>[2x]MKEYHIDEEVGFALPNPQENLPDFYN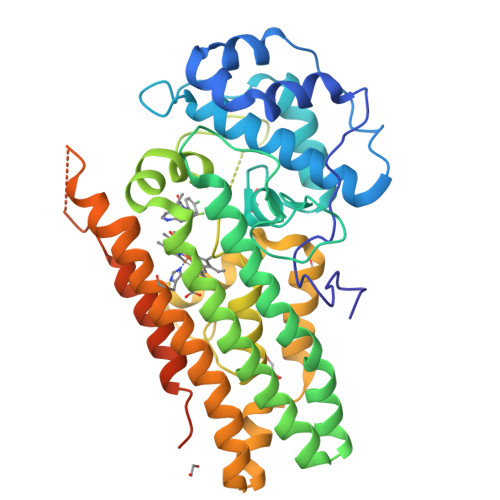DWMFIAKHLPDLIESGQLRERVEKLNMLSIDHLTDHKSQRLARLVLGCITMAYVWGKGHGDVRKVLPRNIAVPYCQLSKKLELPPILVYADCVLANWKKKDPNKPLTYENMDVLFSFRDGDCSKGFFLVSLLVEIAAASAIKVIPTVFKAMQMQERDTLLKALLEIASCLEKALQVFHQIHDHVNPKAFFSVLRIYLSGWKGNPQLSDGLVYEGFWEDPKEFAGGSAGQSSVFQCFDVLLGIQQTAGGGHAAQFLQDMRRYMPPAHRNFLCSLESNPSVREFVLSKGDAGLREAYDACVKALVSLRSYHLQIVTKYILIPASQQPKENKTSEDPSKLEAKGTGGTDLMNFLKTVRSTTEKSLLKEGKGELNSKLEGKPIPNPLLGLDSTRTGHHHHHH>SAAWEDEDLDTDNDNIPDAYEKNGYTIKDSIAVKWNDSFAEQGYKKYVSSYLESNTAGDPYTDYQKASGSIDKAIKLEARDPLVAAYPVVGVGMENLIISTNEHASSDQGKTVSRATTNSKTDANTVGVSISAGYQNGFTGNITTSYSHTTDNSTAVQDSNGESWNTGLSINKGESAYINANVRYYNTGTAPMYKVTPTTNLVLDGETLATIKAQDNQIGNNLSPNETYPKKGLSPLALNTMDQFNARLIPINYDQLKKLDSGKQIKLETTQVSGNYGTKNSQGQIITEGNSWSNYISQIDSVSASIILDTGSQTFERRVAAKEQGNPEDKTPEITIGEAIKKAFSATKNGELLYFNGIPIDESCVELIFDDNTSEIIKEQLKYLDDKKIYNVKLERGMNILIKVPSYFTNFDEYNNFPASWSNIDTKNQDGLQ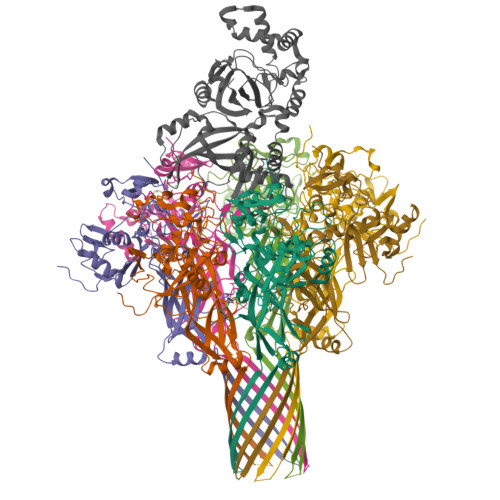SVANKLSGETKIIIPMSKLKPYKRYVFSGYSKDPSTSNSITVNIKSKEQKTDYLVPEKDYTKFSYEFETTGKDSSDIEITLTSSGVIFLDNLSITELNSTPEILKEPEIKVPSDQEILDAHNKYYADIKLDTNTGNTYIDGIYFEPTQTNKEALDYIQKYRVEATLQYSGFKDIGTKDKEIRNYLGDQNQPKTNYINFRSYFTSGENVMTYKKLRIYAVTPDNRELLVLSVN[7x];> GSHMAFIERPEDFLKDKENAIQWEKKEAERVEKNLDTLEKEALELYKKDSEQISNYSQTRQYFYDYQIESNPREKEYKNLRNAISKNKIDKPINVYYFESPEKFAFNKEIRTENQNEISLEKFNELKETIQDKLFKQDGFKDVSLYEPGNGDEKPTPLLIHLKLPKNTGMLPYINSNDVKTLIEQDYSIKIDKIVRIVIEGKQYIKAEASIVNSLDFKDDVSKGDLWGKENYSDWSNKLTPNELADVNDYMRGGYTAINNYLISNGPLNNPNPELDSKVNNIENALKLTPIPSNLIVYRRSGPQEFGLTLTSPEYDFNKIENIDAFKEKWEGKVITYPNFISTSIGSVNMSAFAKRKIILRINIPKDSPGAYLSAIPGYAGEYEVLLNHGSKFKINKVDSYKDGTVTKLILDATLIN> MGSSHHHHHHSQDPNSHMKETPLSNCERRFLLRAIEEKKRLDGRQTYDYRNIRISFGTDYGCCIVELGKTRVLGQVSCELVSPKLNRATEGILFFNLELSQMAAPAFEPGRQSDLLVKLNRLMERCLRNSKCIDTESLCVVAGEKVWQIRVDLHLLNHDGNIIDAASIAAIVALCHFRRPDVSVQGDEVTLYTPEERDP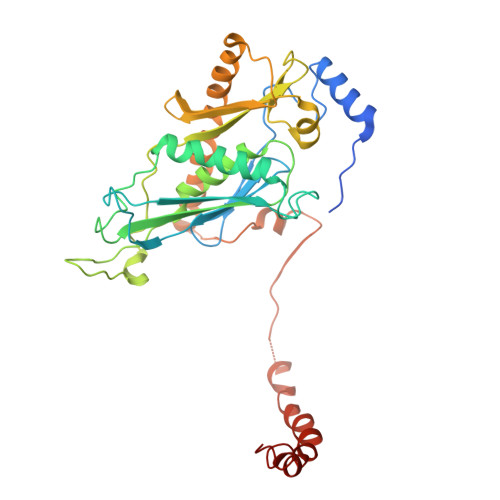VPLSIHHMPICVSFAFFQQGTYLLVDPNEREERVMDGLLVIAMNKHREICTIQSSGGIMLLKDQVLRCSKIAGVKVAEITELILKALENDQKVRKEGGKFGFAESIANQRITAFKMEKAPXXXXXXXXXXXXXXXXXXXXXXXXXXXXXXXXXXXXXXX{4-[2-(5,6-dimethoxypyridin-3-yl)-5-oxo-5,7-dihydro-6H-pyrrolo[3,4-b]pyridin-6-yl]-1H-pyrazol-1-yl}acetonitrile 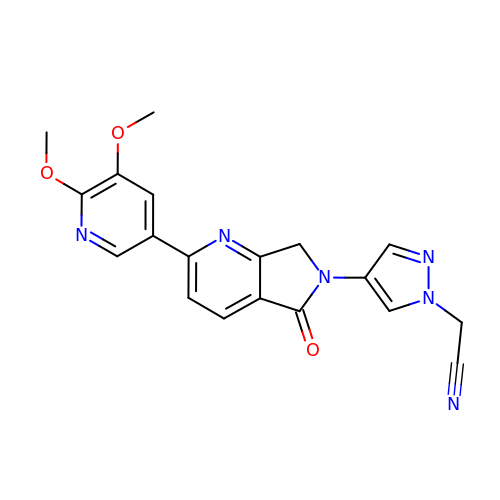| C19 H16 N6 O3 | GJYZEKGSGNPMLK-UHFFFAOYSA-N>MIEQQMDRIVKEMRRQLEMIDKLTTREIEQIELLKRIHDNL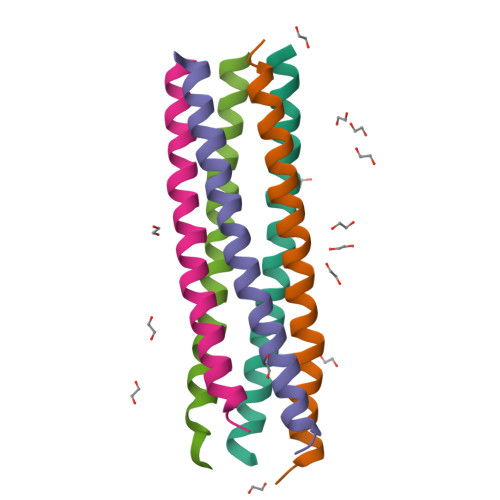ITRPVNVIDMSM[10x]> ANENNQQKIELTVSPENITVYEGEDVKFTVTAKSDSKTTLDFSDL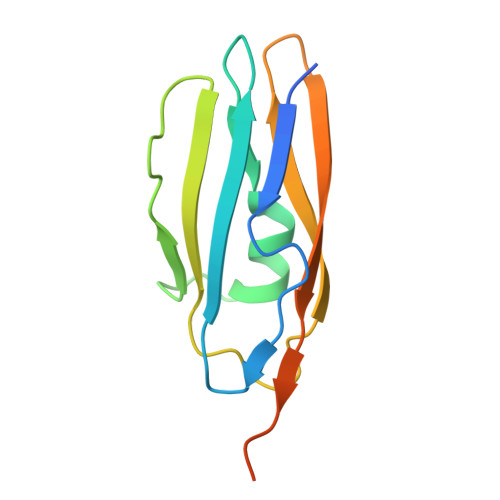LTKYNPSVSDRISTNYKTNTDNHKIAEITIKNLKLNESQTVTLKAKDDSGNVVEKTFTITVQKKEEKQLPSTGGSHHHHHH>[6x]GGGMFNYTVLPSTSLAVGYYYNFLREILEAFNNQKSIQIILERDRTGKPTKTIDYEIKKPYPTIEIRVPQNLASLKKEVLTWNTSEYKQIFINAASRTYPFFLQGEFKEDQILSIFDIPTTLYASYLTIKELFTDSFLKTQNNERKLINKEIRNFERTLSKLIDDTIEEKFYKFTIY

A recent groundbreaking study discovered the ancient origins of the cGAS-STING pathway in bacteria, which play a similar role in the immune system to combat bacteriophage infections. Binding of cGG to bacterial STING causes it to oligomerize into long filaments and activates the nicotinamide adenine dinucleotide (NAD)+ cleavage activity of its fused N-terminal Toll/interleukin-1 receptor (TIR) domain. Depletion of the electron carrier NAD+ eventually leads to bacterial growth arrest or cell death, restricting the replication of invading phages in infected bacteria, a strategy called “abortive infection. In this study, we demonstrated two distinct mechanisms underlying the regulation of bacterial STINGs and a structural basis for cAA recognition and oligomerization.

Through analysis of hundreds of bacterial STINGs, we found that some bacterial STINGs thriving in extreme environment have insertion sequence at the beginning of C-terminal STING domain. We determined the crystal structure of one of the longer bacterial STINGs, Larkinella arboricola STING (LrSTING) to 2.73 Å resolution; the asymmetric unit contains six similar polypeptide chains of LrSTING (root mean square deviation of 0.3 − 0.5 Å for 127 − 149 Cα pairs), which assemble onto three V-shaped dimers with a cGG bound in the central ligand-binding pocket. LrSTING dimers are similar to previously determined cGG-bound bacterial STINGs (r.m.s.d. of 1.3 − 1.9 Å for 185 − 195 Cα pairs), with the exception that LrSTING contains strikingly longer β strands a and b (βa and βb). The longer βa and βb form a continuous β sheet with β1 and β2 and make extensive interactions with βa and βb of the other protomer, forming an additional long lid above the original lid. Superimposition of the three LrSTING dimers in the asymmetric unit revealed that their overall structures are nearly identical, except for significant conformational changes of the additional long lid, suggesting higher structural flexibility as indicated by B-factor values. In contrast, the long lid of LrSTING (chains CD) form one interchain H-bond (K202/T206) and one salt-bridge (R199/D208) at only one end, whereas the long lid of LrSTING (chains EF) does not interact with each other. It is thus suggested that the three different lid conformations of LrSTING are probably snapshots of a dynamic process of lid opening and closing, suggests a regulatory role to control CDN access to the ligand-binding pocket. In summary, these data suggested that the formation of an additional long lid of LrSTING results in autoinhibition, leading to attenuated E. coli toxicity and anti-phage ability. Here we report that dozens of bacterial STINGs contain additional insertion of 14–15 amino acids compared with canonical STINGs and that the insertion sequence correspond to an additional long lid above ligand-binding pocket in LrSTING structure.N-[2-methyl-5-({[3-(4-methyl-1H-imidazol-1-yl)-5-(trifluoromethyl)phenyl]carbonyl}amino)phenyl]isoxazole-5-carboxamide 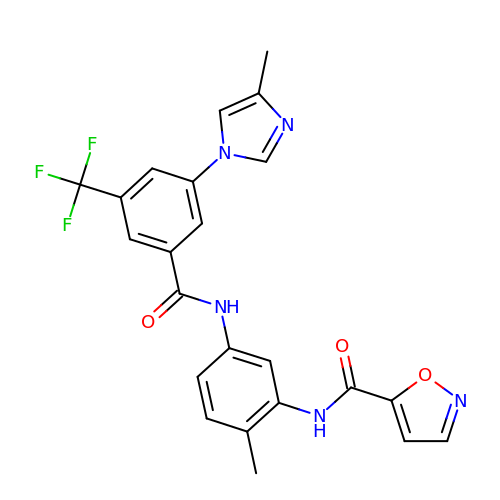| C23 H18 F3 N5 O3 | IYUFHBXMTTXZBE-UHFFFAOYSA-N> MAHHHHHHMTASSDRKAVLITGASRGIGRATAVLAAERGWDVGINYARDAAAAELTAQAVRDAGGRACIVAGDVANEADVVAMFDTVAAAFGRLDALVNNAGIVAPSMPLADMPVDRLRRMFDTNVLGAYLCAREAARRLSTDRGGRGGAIVNVSSIASRLGSPNEYVDYAGSKGAVDSLTIGLAKELGPHGVRVNAVRPGLIETDIHASGGQPGRAARLGAQTPLGRAGEAQEVAEAIVWLLGDTASY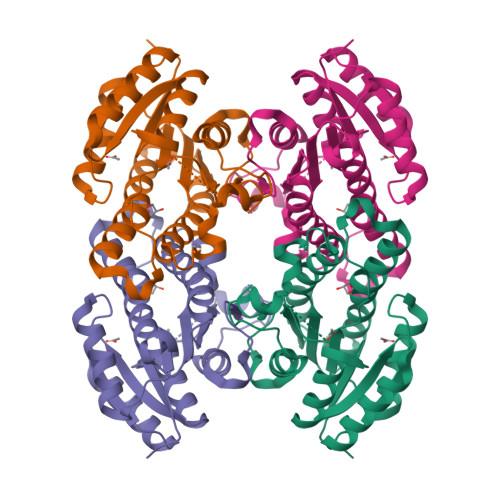TTGALLDVGGGR> TIPHLAIDPFSLDFFDDPYPDQQTLRDAGPVVYLDKWNVYGVARYAEVHAVLNDPTTFCSSRGVGLSDFKKEKPWRPPSLILEADPPAHTRPRAVLSKVLSPATMKTIRDGFAAAADAKVDELLQRGCIDAIADLAEAYPLSVFPDAMGLKQEGREHLLPYAGLVFNAFGPPNELRQTAIERSAPHQAYVNEQCQRPNLAPGGFGACIHAFTDTGEITPDEAPLLVRSLLSAGLDTTVNGIGAAVYCLARFPGELQRLRSDPTLARNAFEEAVRFESPVQTFFRTTTREVELGGAVIGEGEKVLMFLGSANRDPRRWSDPDLYDITRKTSGHVGFGSGVHMCVGQLVARLEGEVMLSAL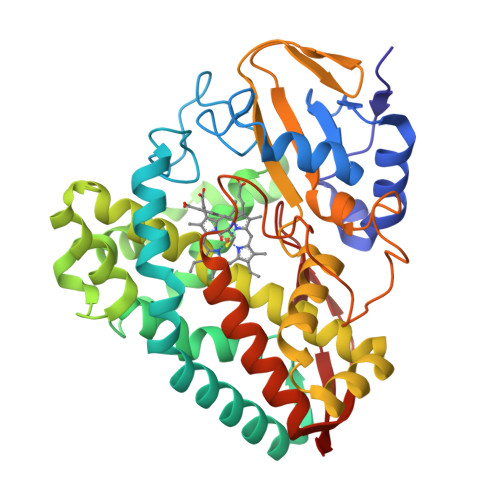ARKVAAIDIDGPVKRRFNNTLRGLESLPVKLTPA>[2x]SNATEELTTVRDACARTLENTARTLHLGASGTEFVAAFRAMTDHWGAARPHDLPLSDVSPDGSPVEYAVDLGGLAPALQFAMEPLTAGVPARDPLAARAIMPLLAGRYGADATRWSALADRLLPDDAHGPHVSMYGAEVRAGAPIRFKAWFYLNVTGPDGAFNLLYSALERMGTTHLW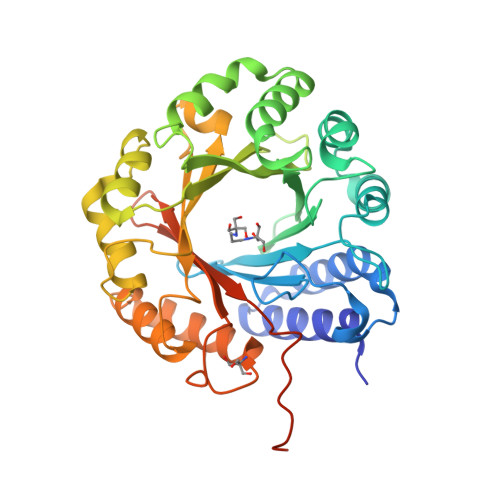PVVQAHVHRAGEDVPFLLSLDLSDDPAARVKVYFRHFAADVEEVAAVLKAYPGFEPGEVRAFCKVMMGGRRRFSDQPAVTCVSLLDAQTFDRTAATLYVPLWTYAEHDGEVRQRVHRTLAAWPEALYRYDSVLAGIAHRGLDAGTGIHNYISWQPGRTRPRMKVYLSPEMHDVTPPPLGVSQQHHLSGQTTARGRTE>[3x]GGGGGGMNLRRRGIVVSFHSNMVTVEDEETGERILCKLRGKFRLQNLKIYVGDRVEYTPDETGSGVIENVLHRKNLLTKPHVANVDQVILVVTVKMPETSTYIIDKFLVL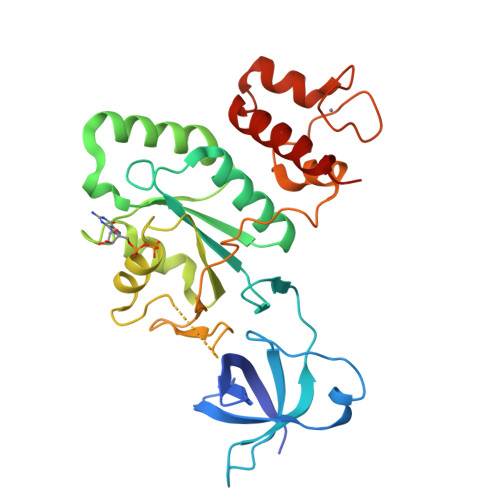AEKNELETVMVINKMDLYDEDDLRKVRELEEIYSGLYPIVKTSAKTGMGIEELKEYLKGKISTMAGLSGVGKSSLLNAINPGLKLRVSEVSEKLQRGRHTTTTAQLLKFDFGGYVVDTPGFANLEINDIEPEELKHYFKEFGDKQCFFSDCNHVDEPECGVKEAVENGEIAESRYENYVKMFYELLGRRKK>[2x]MHHHHHHGSGEGQGPKKQTRLGLEAKKEENLADWYSQVITKSEMIEYHDISGCYILRPWAYAIWEAIKDFFDAEIKKLGVENCYFPMFVSQSALEKEKTHVADFAPEVAWVTRSGKTELAEPIAIRPTSETVMYPAYAKWVQSHRDLPIKLNQWCNVVRWEFKHPQPFLRTREFLWQEGHSAFATMEEAAEEVLQILDLYAQVYEELLAIPVVKGRKTEKEKFAGGDYTTTIEAFISASGRAIQGGTSHHLGQNFSKMFEIVFEDPKIPGEKQFAYQNSWGLTTRTIGVMTMVHGDNMGLVLPPRVAC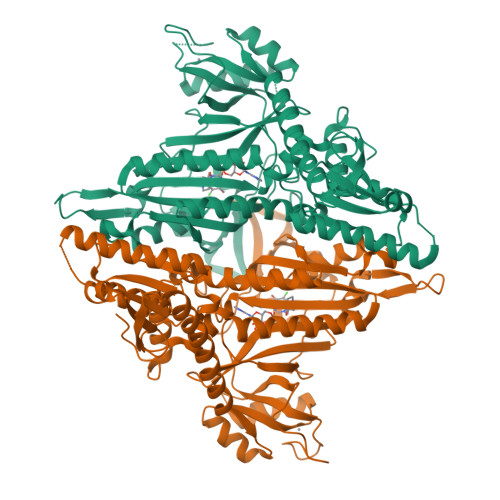VQVVIIPCGITNALSEEDKEALIAKCNDYRRRLLSVNIRVRADLRDNYSPGWKFNHWELKGVPIRLEVGPRDMKSCQFVAVRRDTGEKLTVAENEAETKLQAILEDIQVTLFTRASEDLKTHMVVANTMEDFQKILDSGKIVQIPFCGEIDCEDWIKKTTARDQDLEPGAPSMGAKSLCIPFKPLCELQPGAKCVCGKNPAKYYTLFGRSY> MLSYRHSFHAGNHADVLKHTVQSLIIESLKEKDKPFLYLDTHAGAGRYQLGSEHAERTGKYLEGIARIWQQDDLPAELEAYINVVKHFNRSGQLRYYPGSPLIARQLLREQDSLQLTELHPSDYPLLRSEFQKDSRARVEKADGFQQLKAKLPPVSRRGLILIDPPYEMKTDYQAVVSGIAEGYKRFATGTYALWYPVVLRQQIKRMIHDLEATGIRKILQIELAVLPDSDRRGMTASGMIVINPPWKLEQQMNNVLPWLHSKLVPAGTGHATVSWIVPE

We previously designed adenosine-SAM bisubstrate analogues that contain the SAM cofactor with the S-atom replaced by a N-atom directly linked to an adenosine at the point of nucleophilic attack to mimic the substrate/cofactor bound state. These molecules were used to study the substrate recognition of the m6A MTase RlmJ, the Ribosomal RNA large subunit methyltransferase J that N6-methylates the adenine A2030 of the E. coli 23S rRNA. m6A RNA methyltransferases (MTases) catalyze the transfer of the methyl group from the cofactor S-adenosyl-L-methionine (SAM) to the N6-atom of adenines at specific positions in RNA, releasing the cofactor product S-adenosyl-l-homocysteine (SAH). Two crystal structures of RlmJ in complex with RNA–SAM conjugates were solved and revealed the RNA-specific recognition elements used by RlmJ to clamp the RNA substrate in its active site.

We first investigated whether CA could be accommodated in the RlmJ active site similarly to the SAM cofactor. The crystal structure of RlmJ bound to CA was refined to 2.1 Å and revealed a similar binding mode to that of the natural cofactor. CA and SAH exhibit the same conformations and positioning of both the methionine chain and the adenosine moiety in the active site of RlmJ. Both ligands bind in a pocket lined with RlmJ hydrophobic residues and form hydrogen bonds to conserved residues, namely H19, H42, S100 and D164 via the methionine part and E118 and G144 via the adenosine moiety of CA. The adenine ring is moreover sandwiched between H42 and L119. This structure therefore validates the use of this SAM analogue for the design of RNA–SAM conjugates presented in this paper. Interestingly, H9 swaps conformation from solvent exposed in the RlmJ/CA structure, to buried in the RlmJ/GA* structure, from where it can π-stack with Asub.>MPRKKDQVTKNDDGNQTSDVQTQDFKTAVQPDTNTAQLIKTYSNPKQRGDKGEIIYDGGLSSKLADVVDKTTEPHNADGAVKDGRIAPVKLDLEKQKLDKLKLFETSPFDPLTIKNNQDVVDKLYATQSSSIQEVVPTKTFATELQFGVTSEDMAKIYGAVAAVSKNVNSSVTYEVKRGTHELIKVPTIPHNLVLIQSDNGKHALIKEDLGQWPVETGISLVNQAGVFAVQLANKLGIDKPFVLDAGSNYFTDTSFIDTRKYCTDGLSPREIQKALNRQRAYYDRPELTISENKTLLSQSIIYPDADGNDVSIIFSGAMSHAIFTYAQSQWNKNIIKLDDYIREITLTVPKQYRPRRFKEIEHTHGYVYRELNQGSLLPLVDANLKESSSYYFKKLMSSISNVPVDARTLQSATAALAADTGQAVNRAQHVSMLTNRLTTANAPTVRAITVLTCMFKQFRIGMTYALDPNIMDVAAATCMLLFRPAQSISDEQYRYCLQTMAVFLTNTTYDIVNNDTIDVLKMKLRNQGWPFVERYNAVEIDMSVEPLRSPGQVGRYYNPFNIDPLTKKHVEDRLEEFINQVQVGRFRNASGNAVGTTLAAFLRACRDKTSANWRGYSVLVSRYRSLIPNELFESLRNISGEYNINPQDEHSFFFALAQINADDEFIGAIDKESAEYLDEYATLARDISNSLTLVKAAFGPLERTSGSIINHANNLNKVINHVFADKPLISETMLKILTIDGTTGKDGYRNWLDKLVGHNYPVYVEPVVNIMNFISARFVADSSYFGYTNEIMIMPNHINVPVDDRFGFRDSPFCTSLPRTIMGNDVRRISYNVFSMMEDIDDVISEGFILYDAYFNFSYDIMTTDGVTRLKEDILIVTDTGNDIKPIHFYIYFENRNDKKLRYESKMNVSYRLYIKTPACLLPLSDYMRAQHDYVSPSSSRVYIKDPAVVYTRS[2x];>MANRATSAFLDNPHPVGVNYVDEGSRQFVAVAELLASKLIDSSRESDESNSDVPFVQAYSKFADDNPRHLRVKTGGKMANALTNVIRSYYSINAPAIVPQVEIDRLASKATVSGDMYNSYAIFNSVPIVEVLSPARTTVSIVGSDRADVTMLNTGAGAANITFNFGQIAETVILKGSVPFQLARLNQPMPAARFTYKLRPLDGPFIVVLPVGNPLVISATAATRIQVPLAFNKALVESGFQTAMNDGLFDIQNVNYYSSFDEFIISQYHAQDGINRVSTCVILGLALQAYDQMRRALPVRR[13x];>MDVLSKGSLKELLAHLEKTPLEEAISYRIGTVPYQNVLISRNEYYNQLYPDTTSLIDGVSREGQRNVNGLIMSIISYVVSGSGHYIPNIGFMLLRRSILDILTKHDTGLVTNNLNYGIIARNLTVSKMNCEQRKRMLICFKLLAYKDGNQNDYEIYLNQNIPLKQIAPNFIPGDMRTVIHNQDQLAIVGIPAYRLTQSTELSIRDDNAKSYKLGYVDWYNSNSFLRERSEFNLIRLKDRDTKYGKLNGW[2x];>[6x]MAWVTQAYSSGLSQNSIISLTGNDRTVADGTFNSMIMPRAVIANEREHFMKTRIDKIEHDLNRSAKQEMMDRQSLAEDYNALNLAVGQEIKLDIATQHQLNRLGSAMYKADHERETELTDLINRIRENEVTVNGILENQKAITAAERADLLLEVVASTAKSVSAAGRAAADGSGVVPVFGPSVANGIKVGIDIADSVAEAAIAVKESGIITQLNDVYHAFQSVHVAPNDVIKPAAVVAGTSTELIGNLQAIYSRLRSHSDIGFKKATVGDVIPNSYMIKPVNSTEYASWQLYVIHPVQGSLGLVVQLMGDALTYNVFAQYGNTSASEFGKTVLTGGATNTALEGTKVKFQTKVTAQQALALTMALKDAASMLSQGELIGYFEQYINLALEPDNLSLQDNMHKYHHLLTSQNSPIDWNYHDEEMHKWLDSRKTTNYDAMQKKDGTVIADIHIPKVFNDLRNTTLHCKLEGKQTIAGYTVYEYLIGPWAHYGDIDYSVVVDTLNEETKWYCEVIGIDGHLLIEKSVQHKPEKILELTVNDSGVTSFNGRNHDRLKLKVYVKDSLSVKVFRNWIGINAPRVKTKMFNDHIGVKYDYSHFDKNISPAHLTLTDLGWHTWDQYNAGNWTNIKP;>MLSETELRALKKLSTTTSRVVGDSTLALPSNVKLSKGEVEKIAVTKKEMFDELAQCN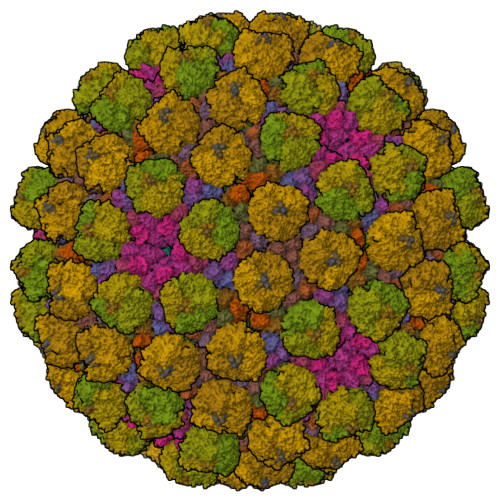LPTIELITREHTFNGDVIRFAAWLFLMNGQKLMIANNVAVRMGMQYATNLAGNNVKITYVTSNNVVKLGHIAAGVLANPYSNKGSGLFITYEYNLISNLIETGKVCVLFITSLSTTASSTNSFAYSTCSVPIENWDFNMIKLTAETSCASLTAMTNLVNSLVPGERTRPVGLYVDIPGVTVTTSASSGSLPLTTIPAVTPLIFSAYTKQVEEVGVINTLYALSYLP[6x]> MSAEITSGDLDQFKQDLQATPAANALQKAVMNNGINATAENTDSKVAMTPTFSIELDTGAVSNQKQSGRCWMFAALNTMRHGIQAQFKIKDFELSQNYTFFWDKFEKSNYFYENVLKTADQPLDSRKVAFLLATPQQDGGQWDMLSALIEKYGIVPKSVMPET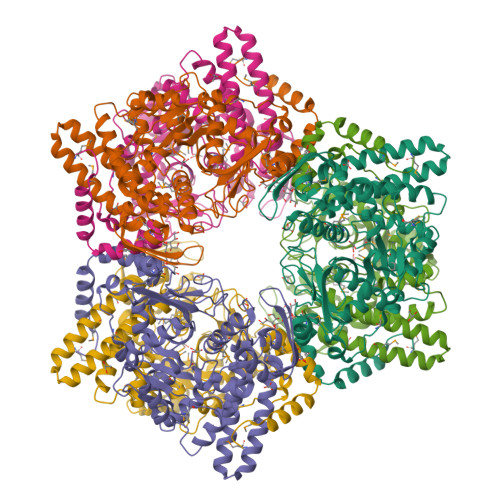YSSSKSNELNGLLNLKLRKDAVTLRKLVADKASDADIEAAKQKMLAEDYRILAYTLGNPPTKFDFEYRDDDKNYHIDRELTPQTFFKKYVGWNLDDYQSIINAPTADKPYKHLYTVEMLGNVVGGREVRHLNLDIDTFKDLAIKQLKAGESVWFGSDVGQSSDRQLGILDTNIYKKDDLFNTDFTMTKAERLDYGESLMTHAMVLTGVDLVDGKPTKWKVENSWGEKVGEKGYFVASDAWFDQFVYQVVISKKYLPAELQDVIKNEYDKPTVLAPWDPMGALA>[2x]AMDFPQQLEACVKQANQALSRFIAPLPFQNTPVVETMQYGALLGGKRLRPFLVYATGHMFGVSTNTLDAPAAAVECIHAYSLIHDDLPAMDDDDLRRGLPTCHVKFGEANAILAGDALQTLAFSILSDADMPEVSDRDRISMISELASASGIAGMCGGQALDLDAEGKHVPLDALERIHRHKTGALIRAAVRLGALSAGDKGRRALPV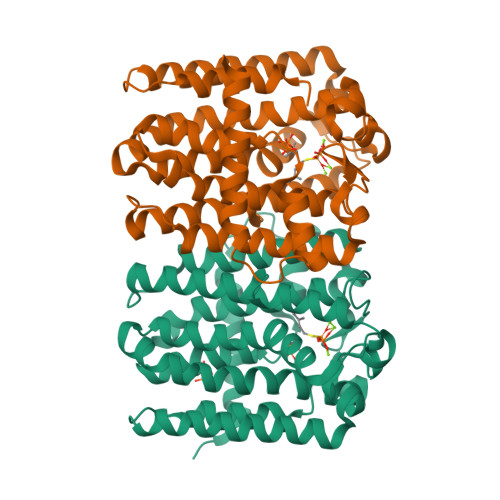LDKYAESIGLAFQVQDDILDVVGDTATLGKRQGADQQLGKSTYPALLGLEQARKKARDLIDDARQSLKQLAEQSLDTSALEALADYIIQRNK(1R,3aS,3bR,5aR,7R,9aS,9bS,11aR)-1-[(2R)-6-fluoro-5-oxohexan-2-yl]-9a,11a-dimethylhexadecahydro-1H-cyclopenta[a]phenanthren-7-yl 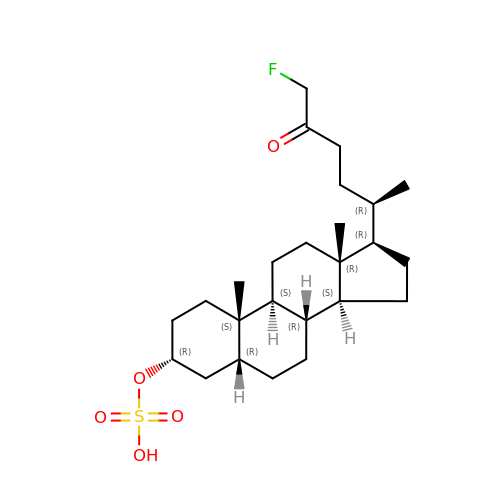hydrogen sulfate (non-preferred name) | C25 H41 F O5 S | MVPISWRWXKQVBV-CIQXVCGBSA-N> MEAEQVWKLWRRVLRDERLQAQLFSATDATHWLSGFSESESKILSVYAQQFDRVKWFVENYQFRLVNSFLNALETGAPLSLRALLHINVDLNAQSKAFLRDRQWRDYGPQVYTYCEDVLGFLAEADELQGYPEILDLMRLERESVRLYRGLVDPESLPADNRYQRTSMARLYETRFALSGWLRQKDQLGLTRLPESTEHVLIYLPTLQARHKFTLINAQAARLYNCLEQPQSAAGLFMLINSDSASVPGSADLALLDRLEQLNAIRKPL;> MPDFVKPAPIGVGIQYNPEILDWFPFEDIQVDILEILLDNIMAPMDGPQIIKPSAQAMIERLGQKFTLLAHSNYGCDFGFSALEETAAVQRHVPLAKMLNSPWVANHCFYGDQSWLDIWSSPIQFSAAEVARCADRAQSLQTLYGMPLAHENAAYYLECPGAEMREAEFLARLVQRSGTFLHLDLHNIYTNHLNLKGFDLKDYMDTLPLDKVISVHLAGGSWHGGLYHDWHDACVPEPVWDLYEDLLSRAQPSAVILEYQGQAHHAQTRIMDASDESMIVRDVQRAQAIWSRYNRHPQERQYGS

The next unusual PTM reaction on TglA-Cys is performed by a complex formed by TglH and TglI, in which the cysteine β-methylene (β-CH2) of TglA-Cys is removed to generate TglA-CysΔCH2. Like MbnB and MbnC, TglH and TglI of the TglHI holoenzyme likely function as a catalytic and recruitment subunit, respectively, to achieve TglA-Cys modification. Here, we report the structures of TglHI in the absence of Fe ions, with two Fe ions, and with three Fe ions (apoTglHI, TglHI-2Fe and TglHI-3Fe, respectively). The interaction with TglI is required for TglH catalytic activity, indicating that the TglHI complex acts as a holoenzyme for 3-thiaGlu generation, akin to MbnBC.

Therefore, E. coli BL21 containing a tglHI plasmid were cultured in LB medium supplemented with 1 mM ammonium ferrous sulfate. This procedure resulted in TglHI crystallizing with iron and structures of TglHI with two or three Fe atoms were determined and named TglHI-2Fe (3.25 Å) and TglHI-3Fe (3.49 Å), respectively. Structural comparison between apoTglHI and TglHI-2Fe revealed that loops L4 (residues 258–275) and L2 (residues 107–126) of TglH are in very different orientations. Loop L4 closes over the active site in the TglHI-2Fe cap whereas loop L2 swings away from the active center. The conformational changes in the loops induced by binding of two Fe ions result in the overall transition of TglH from an open to a closed active site cavity. In addition, the changes upon iron binding enhance the hydrophobicity of the active center with an increase in buried surface area of about 309 Å2 (from ~493 Å2 to ~802 Å2). In the TglHI-2Fe and TglHI-3Fe structures, Fe1 and Fe2 are coordinated by His71, His107, Glu151, Asp184, His216, and Glu258, as well as water molecules. The structural models of TglHI-2Fe and TglHI-3Fe were supported by ICP‒OES, which illustrated that the number of Fe ions per heterodimer of TglHI-2Fe and TglHI-3Fe was 1.50 ± 0.09 and 2.48 ± 0.18, respectively. Structural superposition of TglHI-2Fe and TglHI-3Fe illustrated no significant conformational changes (RMSD: 0.63 Å), implying that the third iron plays a minor role in the TglHI-3Fe structure. In this work, it appears that two Fe ions are sufficient for TglA-Cys modification.>[2x]MEIQEISKLAIEALEDIKGKDIIELDTSKLTSLFQRMIVATGDSNRQVKALANSVQVKLKEAGVDIVGSEGHE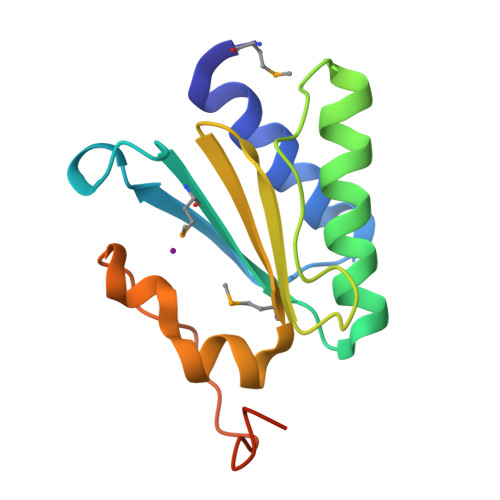SGEWVLVDAGDVVVHVMLPAVRDYYDIEALWGGQKPSFAVGAAKPWSAVLEHHHHHH> GSHMTKYKYTVEESERFNKHGIDLTVYGQVDPSATVVRVSVERGHFQEFFNVRSSYTFYVVSGQGVFYLNSEAVPAGATDLITVPPNTRIHYFGSMEMV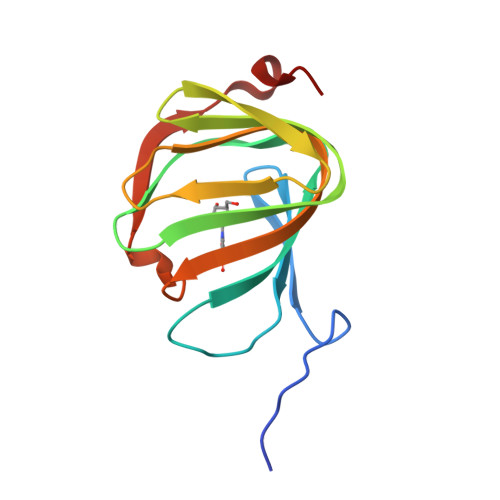LTVAPAFNEQDERHVRFISESESPY> HMNRISWVGEAVKTDGKKSYYKKVCIDAETLEVGDCVSVIPDDSSKPLYLARVTALWEDSSNGQMFHAHWFCAG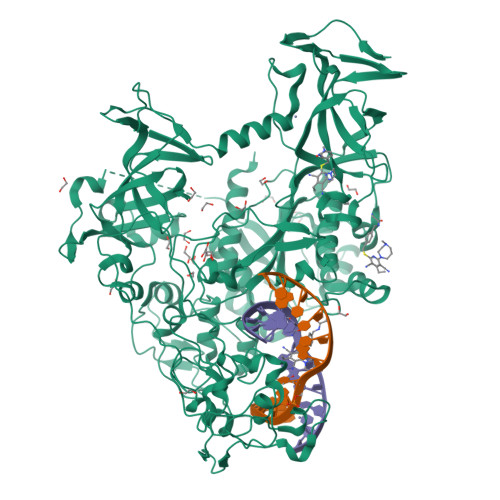TDTVLGATSDPLELFLVDECEDMQLSYIHSKVKVIYKAPSENWAMEGGMDPESLLEGDDGKTYFYQLWYDQDYARFESPPKTQPTEDNKFKFCVSCARLAEMRQKEIPRVLEQLEDLDSRVLYYSATKNGILYRVGDGVYLPPEAFTFNIKLSSPVKRPRKEPVDEDLYPEHYRKYSDYIKGSNLDAPEPYRIGRIKEIFCPKKSNGRPNETDIKIRVNKFYRPENTHKSTPASYHADINLLYWSDEEAVVDFKAVQGRCTVEYGEDLPECVQVYSMGGPNRFYFLEAYNAKSKSFEDPPNHARSPGNKGKGKGKGKGKPKSQACEPSEPEIEIKLPKLRTLDVFSGCGGLSEGFHQAGISDTLWAIEMWDPAAQAFRLNNPGSTVFTEDCNILLKLVMAGETTNSRGQRLPQKGDVEMLCGGPPCQGFSGMNRFNSRTYSKFKNSLVVSFLSYCDYYRPRFFLLENVRNFVSFKRSMVLKLTLRCLVRMGYQCTFGVLQAGQYGVAQTRRRAIILAAAPGEKLPLFPEPLHVFAPRACQLSVVVDDKKFVSNITRLSSGPFRTITVRDTMSDLPEVRNGASALEISYNGEPQSWFQRQLRGAQYQPILRDHICKDMSALVAARMRHIPLAPGSDWRDLPNIEVRLSDGTMARKLRYTHHDRKNGRSSSGALRGVCSCVEAGKACDPAARQFNTLIPWCLPHTGNRHNHWAGLYGRLEWDGFFSTTVTNPEPMGKQGRVLHPEQHRVVSVRECARSQGFPDTYRLFGNILDKHRQVGNAVPPPLAKAIGLEIKLCMLAKA> MADKNYLHTAYANSADGTDGFTTVYPNLNLLVNSSAKNKEGFFKNFDKVENGYGEVTMKGTNAWVNKDLGEGFSIQPINYKPGDKY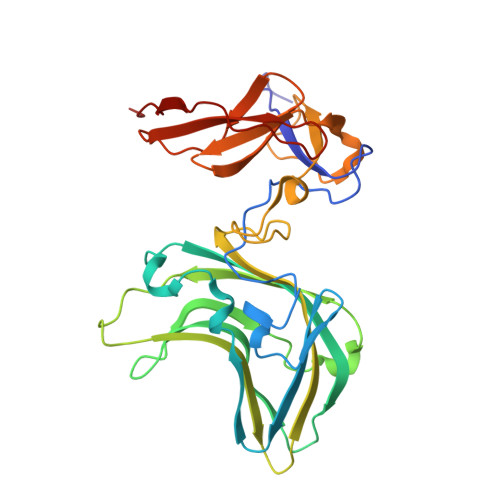TMSVDVMFTSWNVPAGTTISAFWMRQRYTENSWKEICTIDLPKDPSKMLNQWIRITQTSTIPPYEDPSVGTQAILNVGFFGQQEGSFTIRVRNPKQELGSIATPYMPSASEVTTADWPKFVGTYVDTNPVSSTVSSKYDWDEMKYRVYLDGTPVGGSKLLSFDLENLKAGTSYNVQVSQINGNVESDKSESVAFKTTLPK> MKTTPLVHVASVEKGRSYEDFQKVYNAIALKLREDDEYDNYIGYGPVLVRLAWHTSGTWDKHDNTGGSYGGTYRFKKEFNDPWNAGLQNGFKFLEPIHKEFPWISSGDLFSLGGVTAVQEMQGPKIPWRCGRVDTPEDTTPDNGRLPDADKDADYVRTFFQRLNMNDREVVALMGAHALGKTHLKNSGYEGPWGAANNVFTNEFYLNLLN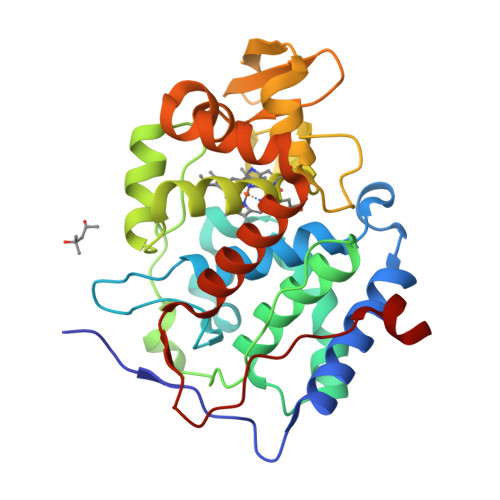EDWKLEKNDANNEQWDSKSGYMMLPTDYSLIQDPKYLSIVKEYANDQDKFFKDFSKAFEKLLENGITFPKDAPSPFIFKTLEEQGL> MGVISDAYRLKYTFGVDFGTSYVKYGPITLNEPKMVQTRGLFLRDLPESVKMRIPPDVLARGLVVGDEEVRKYLSSVRDVQRNLKYPLKDGVARRDDEEAWRVLKELARYTLAQFPVSDPEFAGWLVAVALSALAPDYMYKAIFDIYDELASEFKIYAVTILPQPLAVAIAENAVNCVIVEGGHGNIQVAPISFALIREGLVALNRGGAEANAITREILKDIGYSDIAREEYAVEVVKRAVGLVPRRLKEA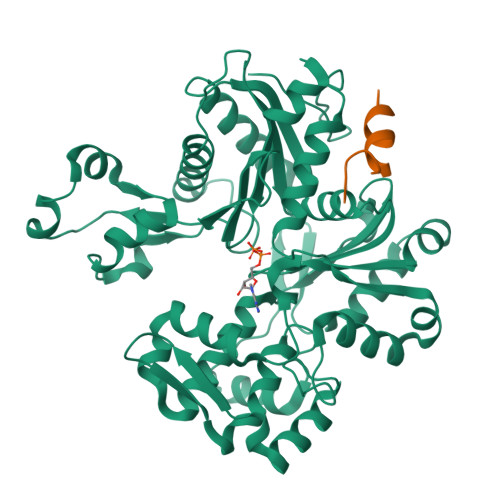IRAAKSDPDRFVTKVRLSPVVEVEIPREYAWTRFLIGEIVFDPNHEEIKSYIEQSRLRIENAVIGDVTLYGEMDVASAIITSLRNVSVEIQERVASQIILSGGAFSWRVPPGMEDVAADSVTRVKIALEEKSPALASKVEVRLVSEPQYSVWRGAVIYGYALPLSLEWSDTTREGWRFPRR;> GGIGENEWVKILRSKR>VTTTATLTYPFHDWSQELSPRYAQLRASDAPVCPVVSEGTGDPLWLVTRYATAVKLLEDSRFSSEAAQASGAPRQEPVELRAPGTRGDAIAMLREAGLRSVLADGLGPRAVRRHQGWINDLAETLMSELASREGTFDLAADFVEPLSSALVSRTLLGELSADERDLLAHCADTGLRFCGVTHEEQVHAFTQMHEFFLEHARRLAGTPGEHLLKLIAEAPVDQGPLSDEALAEAGSLLVVAGFPTSSGFLCGALLTLLRHPDAVQELHAHPERVPSAVEELLRYTPLSTGSVKRMATEDLEIDGVRIKAGEVVMVSLEAVNHDPDAFEDPDVFRPGREGPMHFGFGRGRHFCPGNRLARCVIEATVRAVARR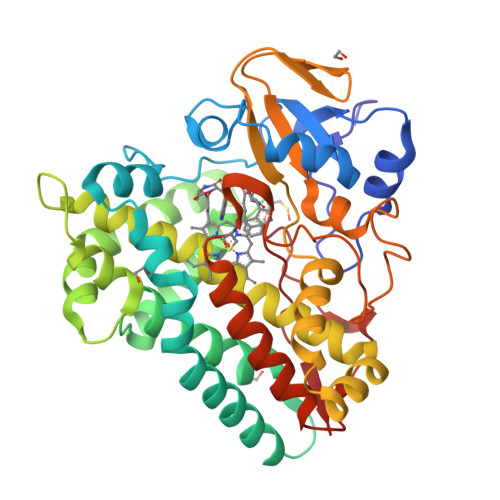PGLRLAVAPEEISWHEGLFFRRPRAIPATW[2x]>[2x]MKHHHHHHDEIISELRELCLNYIEQDERLSRQKLNFLGQREPRMVLIEGLKLLSRCIEIDSADKSGCTHNHDDKSVETILVESGIVCPGLPLIIPDGYKLIDNSLILLECFVRSTPASFEKKFIEATNKLACIREDLAVAGVTLVPIVDGRCDYDNSFMPEWANFKFRDLLFKLLEYSNQDEKVFEESEYFRLCESLKTTIDKR

The endonuclease domain is at the N-terminus of the L protein, a multifunctional protein that includes the RNA-dependent RNA polymerase. The synthesis of mRNA in arenaviruses is a process that is primed by capped nucleotides that are ‘stolen’ from the cellular mRNA by the endonuclease domain in cooperation with other domains of the L protein. The L protein cleaves and snatches the native cellular mRNA cap structure through its endonuclease domain after ∼11 nucleotides, and uses it as a primer sequence for the RdRp domain of the L protein to synthesize the viral mRNA. The catalytic centre of the ENDO resides in the N-terminal part around Asp88 and should contain two Mg2+ (or Mn2+) ions, which are critical for the RNA-cleavage mechanism.

In this study, we decided to assess the impact of a key residue within the catalytic site but a priori not involved in the mechanism. For this, we mutated a conserved aspartate to alanine (D118A). From a structural point of view, we confirmed by crystallography that the mutation has no effect on the overall LCMV endonuclease structure, as preliminarily shown by the study of the thermal stability of ENDO-D118A by DSF. D88A is a mutation of the key residue supposedly involved in bivalent metal-ion coordination, while D118A is a mutation of a conserved residue distant from the active site in the vicinity of the catalytic pocket. (ii) Asp118 makes no direct or indirect interactions with the ions and has virtually no influence on the stability of the protein. This result was confirmed by our structural study (see §3.2). Any change in the hydration shell of proteins owing to changes in their structure affects the thermophoretic movement, which is used to determine binding affinities with high accuracy and sensitivity. The results summarized in Table 2 show that the affinities of ENDO-WT and ENDO-D118A for DPBA (1) are in the same (micromolar) range. ENDO-WT and ENDO-D118A displayed affinities in the low-micromolar range, while no interaction was detected for ENDO-D88A, confirming the earlier results.> GPGTRTGRLKKPFVKVEDMSQLYRPFYLQLTNMPFINYSIQKPCSPFDVDKPSSMQKQTQVKLRIQTDGDKYG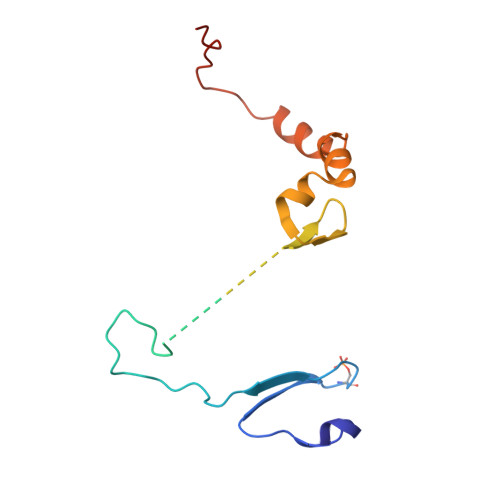GTSIQLQLKEKKKKGYCECCLQKYEDLETHLLSEQHRNFAQSNQYQVVDDIVSKLVFDFVEYEKDTPKKKR Many NLR proteins nucleate the “inflammasome”—a large macromolecular complex that triggers inflammatory cell death and cytokine secretion in response to microbial or danger-associated ligands. Like many other supramolecular assemblies in the human innate immune system, the inflammasome complex relies on homotypic and heterotypic interactions between the death domains (DDs) to initiate, amplify, and propagate pyroptotic signaling. Inflammasome sensor NLRs can be grouped into two categories based on their DDs: PYRIN domain (PYD) and caspase activation and recruitment domain (CARD), both domains were found to form filamentous complexes to initiate the inflammasome formation. Extending this analysis, we also found that specific type II interface motifs directly dictate the compatibility of heterotypic pairwise CARD-CARD interactions among NLRP1, CARD8, NLRC4, ASC, and CASP1.

To test this, we solved the structures of recombinant NLRP1-CARD and CARD8-CARD filaments using cryo-EM, both at 3.7 Å with Gold standard FSC = 0.143, without masking. NLRP1-CARD filaments are relatively flexible and adopt multiple helical organizations in vitro, as evidenced by heterogeneous 2D and 3D classes observed during structural analysis using RELION 3.0. Trimming of the last eight a.a. (1466–1473) helped stabilize the homogenous form of NLRP1-CARD single filament. This conformation was subsequently verified to be a signaling-competent confirmation based on functional experiments using 293T-ASC-GFP cells (see below). Importantly, the resolved CARD filament density fits snugly into the lower resolution model of NLRP1-FIINDUPA-CARD filament based on negative stain EM, matching the shape and dimensions of the inner layer almost perfectly. NLRP1-CARD filaments demonstrate a balanced charge distribution on its axial surface, similar to previously published DD complexes. In the NLRP1-CARD complex, two positively charged histidine residues (His1454 and His1452) extend from the Type IIb surface and interact with negatively charged residues, Asp1437 and Ser1435 on the Type IIa surface. In other words, NLRP1-CARD uses the HPH motif on its Type IIb surface to preferentially engage ASC-CARD and disfavor CASP1-CARD. Thus, NLRP1 requires endogenous ASC for inflammasome activation in human cells, whereas CARD8 can directly activate caspase-1 independently of ASC.

>GPGDYKDDDDKDAPQLLHFVDQYREQLIARVTSVEVVLDKLHGQVLSQEQYERVLAENTRPSQMRKLFSLSQSWDRKCKDGLYQALKETHPHLIMELWEKGSKK[12x]>MFGRKKGDVIDAGAELERAEQERIEGEYGASELASERRPHTPGARTLLMVLLCVIAVVLVTLSYKAYKVRGVVEDDDAQPQQVVRQVIPGYTPRPIRPEPENVPEPPQPTTSVPAIQPAPVTQPVRPQPTGPREKTPYELARERMLRSGLTAGSGGGEDLPRPQGGDVPAGGLMGGGGGGGELAEKLQPMRLSGSSAGRLGNRDMLITQGTQLDCVLETRLVTTQPGMTTCHLTRDVYSTSGRVVLLDRGSKVVGFYQGGLRQGQARIFVQWSRIETPSGVVINLDSPGTGPLGEAGLGGWIDRHFWERFGGAIMISLIGDLGDWASRQGSRQGDNSIQFSNTANGVESAAAEALRNSINIPPTLYKNQGERVNILVARDLDFSDVYSLESIPTK[16x];>MKKLAIVALLASLHAVPALALDVPSSSRYDHRIRYVTYNPADVVQVDTVLGVATHIMLEEGEQYLTHAFGDSEAYAFARKGRHIFIKPQAELANTNLIVVTDRRSYKFRLQMRNDRNGAMYELAFRYPDTQARQTREANARAAVEAAFEQRVGAYYNLKYMMSGDKDIAPVNAWDDGRFTYFKFSANADLPSIYFVDAEGNESLVPRTTVGSSNNIIAVHKVNPKWMIRLGNRALAIFNEAYDPNGVPNDTGTASPAVRRVNKGGN[16x];>MKTIIFAILMTGLLSACASAPKPKQPSDFNREPVNKTVPVEIQRGAL[14x]

Conjugative type IV secretion systems (T4SS) mediate bacterial conjugation, a process that enables the unidirectional exchange of genetic materials between a donor and a recipient bacterial cell. Bacterial conjugation is the primary means by which antibiotic resistance genes spread among bacterial populations. The recent cryo-electron microscopy (cryo-EM) structure of the conjugative Type 4 Secretion System (T4SS) encoded by the plasmid R388 revealed that the remaining VirB proteins form a large assembly organised into four sub-complexes: the outer membrane core complex (OMCC), the stalk, the arches and the inner membrane complex (IMC). Previously, we solved the cryo-electron microscopy (cryo-EM) structure of a conjugative T4SS. In this article, based on additional data, we present a more complete T4SS cryo-EM structure than that published earlier.

Further analysis employing 3D classification (Fig. EV1) reveals a degree of heterogeneity in the positioning of the two extra TrwF/VirB9NTD-TrwE/VirB10NTD sub-complexes within the I-layer. We obtained three distinct OMCC structures, each characterised by a unique arrangement of the two extra sub-complexes in the I-layer. Aligning the structures of these three I-layer conformations using the O-layer as the reference underscores how the variability in the positions of the two extra I-layer complexes impacts the overall I-layer structure. Although the structure of each complex forming the I-layer do not change significantly (RMSD of 1.06 Å), a shift between corresponding complexes in the superposition of conformations A and B or A and C is observed. In both, this shift changes in magnitude, being maximal in the superposition involving the second extra sub-complex (that in orange in Fig. 2C i.e. complex 10 in the A versus B superposition and complex 11 in the A versus C superposition) and, intriguingly, being minimal in the complexes opposite (complex 2 in the A versus B superposition and complex 3 in the A versus C superposition). Thus, the insertion of extra complexes occurs at various positions in the I-layer, resulting in structural adjustments that propagate over the entire I-layer.>[2x]SEPQDDDYLYCEMCQNFFIDSCAAHGPPTFVKDSAVDKGHPNRSALSLPPGLRIGPSGIPQAGLGVWNEASDLPLGLHFGPYEGR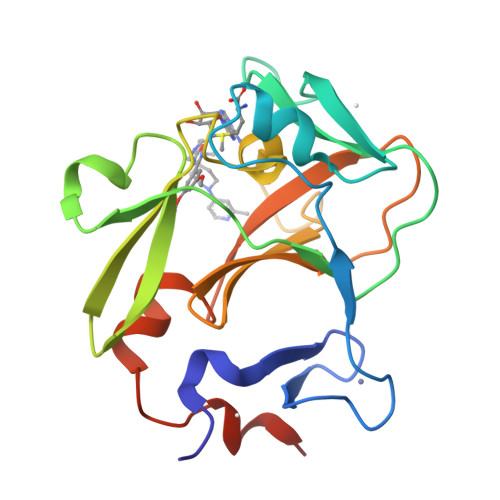ITEDEEAANNGYSWLITKGRNCYEYVDGKDKSWANWMRYVNCARDDEEQNLVAFQYHRQIFYRTCRVIRPGCELLVWYGDEYGQELGIKWGSKWKKELMAGREPKP> MDELGIPVYKRGFPEHLLRGYEFIIDVGTKIESVGGRHDVTKIPEMNAYDIKQESIRTALWYNPIRNDGFVLPRVLDITLRGYDERRAVVESTRHKSFHTNDQWVQWMMKDSMDAQPLKVGLDDQSRNVAHSLHNCVVKIDSKKADTMSYHVEPIEDASKGCLHTRTMMWNHLVRIETFHAAQEVAYTLKPTYDIVVHAERRDRSQPFRPGDQTLINFGRGQKVAMNHNSYDKMVEGLTHLVIRGKTPEVIRDDIASLDEICNRWIQSRHDPGEIKAYELCKILSTIGRKVLDREKEPEDEANLSIRFQEAIDNKFRQHDPERLKIFEHRNQRRDEDRFYILLMIAASDTFNTRVWWSNPYPCLRGTLIASETKLGDVYSMMRSWYDWSVRPTYTPYEKTREQEKYIYGRVNLFDFVAEPGIKIVHWEYRLNHSTREITYAQGNPCDLYPEDDDVIVTKFDDVAYGQMINEMINGGWNQEQFKMHKILKSEGNVLTIDFEKDAKLTTNEGVTMP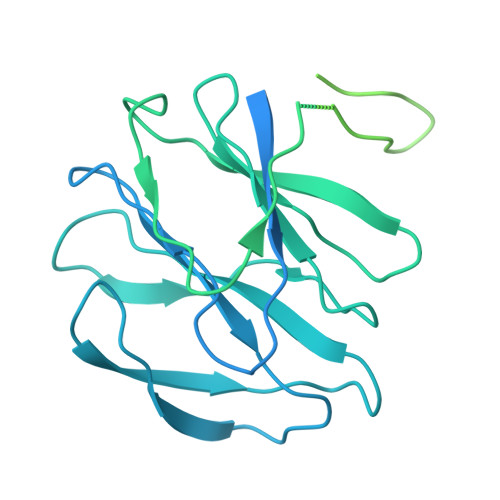EYFNKWIIAPMFNAKLRIKHEEIAQRQSDDPMVKRTLSPITADPIELQRLTLARFYDIRPALRGQALSRQQAQSTYDEEISKQRDY>IRCFITPDITSKDCPNGHVCYTKTWCDAFCSIRGKRVDLGCAATCPTVKTGVDIQCCSTDNCNPFPTRKRP[4x];>[2x]YM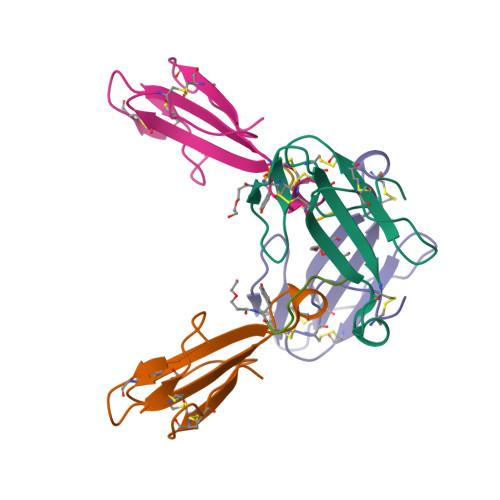WDGWYM>[3x]MVSKAARRRRAAPRQQQRQQSNRASNQPRRRR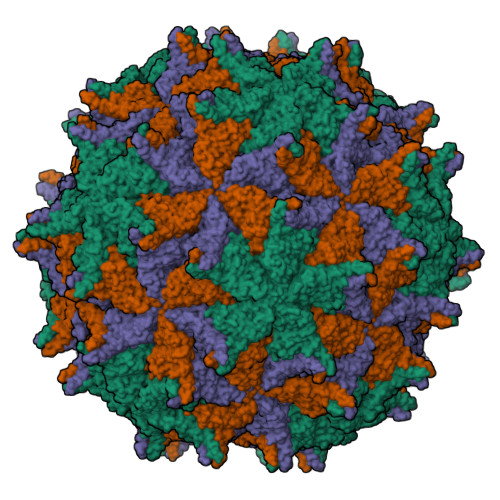ARRTRRQQRMAATNNMLKMSAPGLDFLKCAFASPDFSTDPGKGIPDKFQGLVLPKKHCLTQSITFTPGKQTMLLVAPIPGIACLKAEANVGASFSGVPLASVEFPGFDQLFGTSATDTAANVTAFRYASMAAGVYPTSNLMQFAGSIQVYKIPLKQVLNSYSQTVATVPPTNLAQNTIAIDGLEALDALPNNNYSGSFIEGCYSQSVCNEPEFEFHPIMEGYASVPPANVTNAQASMFTNLTFSGARYTGLGDMDAIAILVTTPTGAVNTAVLKVWACVEYRPNPNSTLYEFARESPANDEYALAAYRKIARDIPIAVACKDN;>ATFWERVRSILKSGLNFASTIPGPVGVAATGIKGIIETIGSLWV[3x]> MGEVVRLTNSSTGGPVFVYVKDGKIIRMTPMDFDDAVDAPSWKIEARGKTFTPPRKTSIAPYTAGFKSMIYSDLRIPYPMKRKSFDPNGERNPQLRGAGLSKQDPWSDYERISWDEATDIVVAEINRIKHAYGPSAILSTPSSHHMWGNVGYRHSTYFRFMNMMGFTYADHNPDSWEGWHWGGMHMWGFSWRLGNPEQYDLLEDGLKHAEMIVFWSSDPETNSGIYAGFESNIRRQWLKDLGVDFVFIDPHMNHTARLVADKWFSPKIGTDHALSFAIAYTWLKEDSYDKEYVAANAHGFEEWADYVLGKTDGTPKTCEWAEEESGVPACEIRALARQWAKKNTYLAAGGLGGWGGACRASHGIEWARGMIALATMQGMGKPGSNMWSTTQGVPLDYEFYFPGYAEGGISGDCENSAAGFKFAWRMFDGKTTFPSPSNLNTSAGQHIPRLKIPECIMGGKFQWSGKGFAGGDISHQLHQYEYPAPGYSKIKMFWKYGGPHLGTMTATNRYAKMYTHDSLEFVVSQSIWFEGEVPFADIILPACTNFERWDISEFANCSGYIPDNYQLCNHRVISLQAKCIEPVGESMSDYEIYRLFAKKLNIEEMFSEGKDELAWCEQYFNATDMPKYMTWDEFFK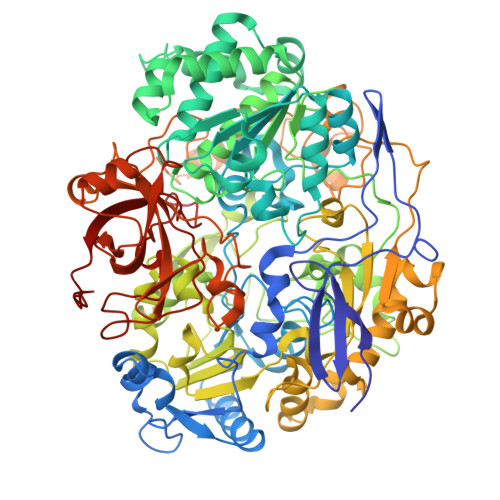KGYFVVPDNPNRKKTVALRWFAEGREKDTPDWGPRLNNQVCRKGLQTTTGKVEFIATSLKNFEEQGYIDEHRPSMHTYVPAWESQKHSPLAVKYPLGMLSPHPRFSMHTMGDGKNSYMNYIKDHRVEVDGYKYWIMRVNSIDAEARGIKNGDLIRAYNDRGSVILAAQVTECLQPGTVHSYESCAVYDPLGTAGKSADRGGCINILTPDRYISKYACGMANNTALVEIEKWDGDKYEIY> QDSTQNLIPAPSLLTVPLQPDFRSDQFRGRWYVVGLAGNAVQKKTEGSFTMYSTIYELQENNSYNVTSILVRDQDQGCRYWI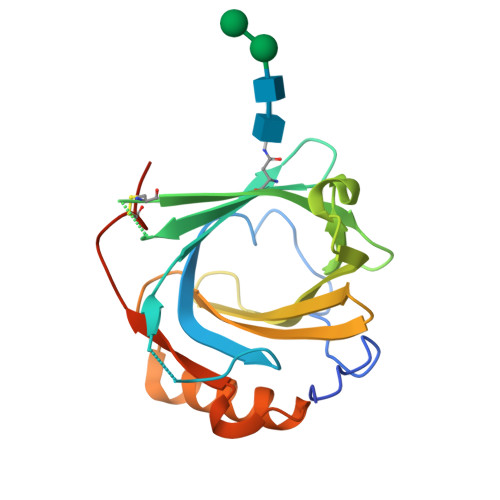RTFVPSSRAGQFTLGNMHRYPQVQSYNVQVATTDYNQFAMVFFRKTSENKQYFKITLYGRTKELSPELKERFTRFAKSLGLKDDNIIFSVPTDQCIDNSAWSHPQFEK>[3x]MFEEINDFETAFKRLLNEVLEFDLQNPLKDVKKVLCIEPHPDDCVIGMGGTIKRLTDRGIEVIYICMTDGYMGTTDENITGHELAQIRRKEEEESAKMLGVKKIYWLNYRDTELPYSREVRKDLVKIIRKEKPDGVFLPDPWLPYEAHPDHRATGFLALDAVAFSPLPNFSNIDLDIGLKPHSVSFIGLYYTSRPNYFVDITDVMDLKLKAIRAHK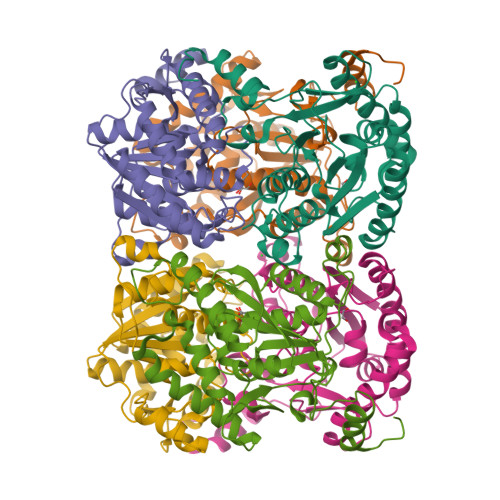SQFPDDIWETWEPFLRTVALYYGQKAGVKYAEGFRIMPGLFYHITPFAELI>AEVVPFNGKGTKASIKFQTMVNWLCENRVFTEDKWKLVDFNQYTLLSSSHSGSFQIQSALKLAIYKATNLVPTSTFLLHADFEQVMCIKDNKIVKLLLCQNYDPLLVGQHVLKWIDKKCGKKNTLWFYGPPSTGKTNLAMAIAKSVPVYGMVNWNNENFPFNDVAGKSLVVWDEGIIKSTIVEAAKAILGGQPTRVDQKMRGSVAVPGVPVVITSNGDITFVVSGNTTTTVHAKALKERMVKLNFTVRCSPDMGLLTEADVQQWLTWCNAQSWDHYENWAINYTFDFPGINADALHPDLQTT[12x]

The main replication protein NS1 plays a critical role in cell cycle arrest, transactivation of viral and host genes, and replication and package of B19V genome. Based on its similarity to other parvoviral replication proteins, such as Rep72 of the adeno-associated virus (AAV), NS1 is predicted to contain one nuclease domain (Nuc, aa 1–176), one oligomerization domain (OD, aa 201–270), one SF3 helicase domain (SF3 HD, aa 271–501), and one zinc-binding domain (ZnD, aa 571–671). The SF3 HD domain of NS1 belongs to the SF3 helicase superfamily, which unwinds DNA with 3′→5′ polarity. Totally, four cryo-electron microscopy (cryo-EM) structures were determined, which revealed the detailed mechanisms for ATP binding and hydrolysis and DNA binding and unwinding by NS1.

Based on these observations, we constructed and purified the NS1_200-501 protein, which is composed of the OD and SF3 HD domains. To further verify the assembly of NS1_200-501, we also performed cryo-EM study and solved one NS1_200-501/AMPPNP complex at an overall resolution of 3.5 Å. In the complex structure, NS1_200-501 assembles as dodecamer. Indicated by the low RMSD value (0.7 Å), the conformation and assembly of the NS1_200-501/AMPPNP complex are very similar to that of the NS1_2-570/AMPPNP structure. Like NS1_2-570, the size-exclusion chromatography profile suggests that NS1_200-501 exists as dodecamer. Although no DNA unwinding activity is observed for the K334A mutant, WT NS1_200-501 can efficiently unwind the DNA. The DNA unwinding activity of WT NS1_200-501 is comparable to that of WT NS1_2-570.> DCPDGWSSTKSYCYRPFKEKKTWEEAERFCTEQEKEAHLVSMENRLEAVFVDMVMENNFENKIYRSWIGLKIENKGQRSNLEWSDGSSISYENLYEPYMEKCFLMDHQSGLPKWHTADCEEKNVFMCKFQLPR;> DFRCPTTWSASKLYCYKPFKEKKTWIEAERFCAKQAENGHLVSIGSAAEADFLDLVIVVNFDKQRYRAWTGLTERNLKWTNGASVSYENLYEPYIRKCFVVQPWEGKSKWYKADCEEKNAFLCKFPKPH;> FNCLPGWSAYDQHCYQAFNEPKTWDEAERFCTEQAKRGHLVSIGSDGEADFVAQLVTNNIKRPELYVWIGLRDRRKEQQCSSEWSMSASIIYVNWNTGESQMCQGLARWTGFRKWDYSDCQAKNPFVCKFSSEC;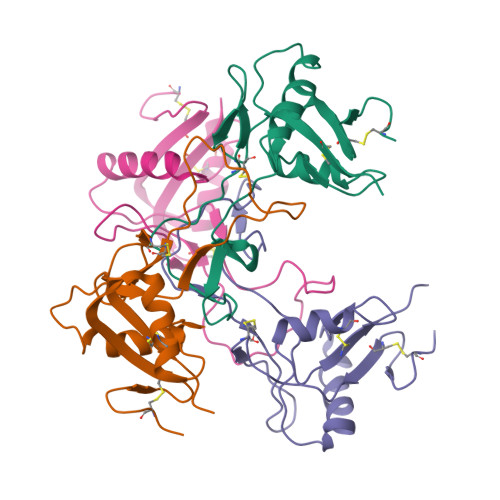> CPLHWSSYNGYCYRVFSELKTWEDAESFCYAQHKGSRLASIHSREEEAFVGKLASQTLKYTSMWLGLNNAWAACKWEWSDDAKLDYKVWLRRAYCAVMVVKTDRIFWYNRGCEKTVSFLCKFYS>[4x]MDVRTLAVGKAHLEALLATRKMTLEHLQDVRHDATQVYFDGLEHLQNVAQYLAIPLSEFFVGQTQSDLDDGVKIARRNGGFKREEIRGGVHYY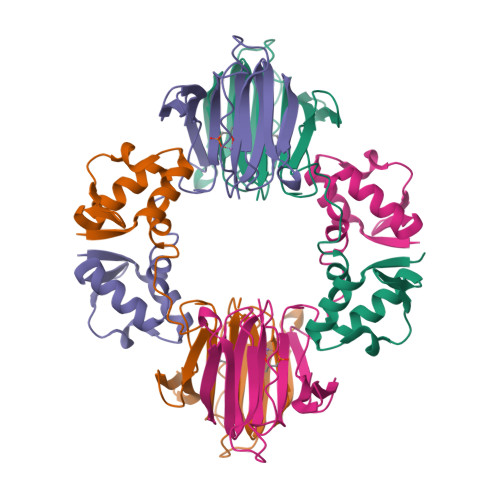TYEHLVTTNQDPGLMALRLDLHSDDEQPLRLNGGHGSREIVYVTRGAVRVRWVGDNDELKEDVLNEGDSIFILPNVPHSFTNHVGGAKSEIIAINYG>GIDPFTMTPSEDFVVTDRGGIVENSHRVHAAVVDAKGRLLYALGNPTRMTLARSAAKPAQALAILETEGVAGYGFDDADIALMCASHSSEDRHIARTRAMLSKIKAEEADLRCGGHPSLSEMVNRSWIKQDFIPTAVCSNCSGKHVGMLAGARAIGAGTDGYHLPDHPMQGRVKRTVAELCDLDAGDVEWGTDGANLPTPAFPLDRLGRIYAKLASAADGSDAGEGQSTRCAALAHIFRAMARHPEMVAGEGRYCTMLMRAFDGALVGKLGADASYAIGVRASDATRQLGTDGALGISVKIEDGNLEMLYAVVTELLERLGIGSPDVRSQLASFHHPQ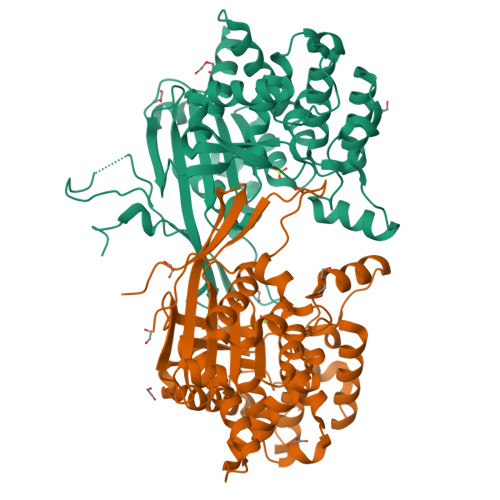RVNTMGVTTGGVSFPFKLRGSKSNVDDPRLAAVAR[2x]>[2x]MSQRITIDPVTRIEGH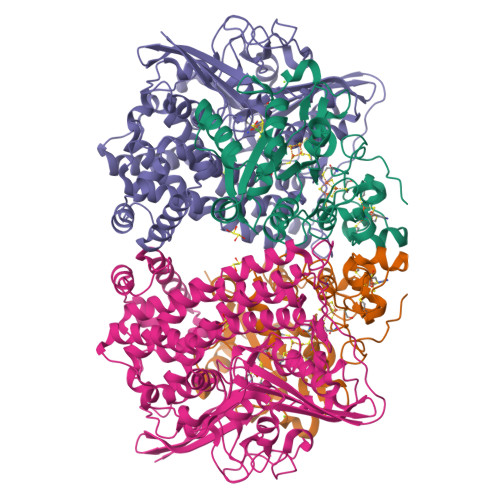LRIDCEIENGVVSKAWASGTMWRGMEEIVKNRDPRDAWMIVQRICGVCTTTHALSSVRAAESALNIDVPVNAQYIRNIILAAHTTHDHIVHFYQLSALDWVDITSALQADPTKASEMLKGVSTWHLNSPEEFTKVQNKIKDLVASGQLGIFANGYWGHPAMKLPPEVNLIAVAHYLQALECQRDANRVVALLGGKTPHIQNLAVGGVANPINLDGLGVLNLERLMYIKSFIDKLSDFVEQVYKVDTAVIAAFYPEWLTRGKGAVNYLSVPEFPTDSKNGSFLFPGGYIENADLSSYRPITSHSDEYLIKGIQESAKHSWYKDEAPQAPWEGTTIPAYDGWSDDGKYSWVKSPTFYGKTVEVGPLANMLVKLAAGRESTQNKLNEIVAIYQKLTGNTLEVAQLHSTLGRIIGRTVHCCELQDILQNQYSALITNIGKGDHTTFVKPNIPATGEFKGVGFLEAPRGMLSHWMVIKDGIISNYQAVVPSTWNSGPRNFNDDVGPYEQSLVGTPVADPNKPLEVVRTIHSFDPCMACAVH;>MEMAESVTNPQRPPVIWIGAQECTGCTESLLRATHPTVENLVLETISLEYHEVLSAAFGHQVEENKHNALEKYKGQYVLVVDGSIPLKDNGIYCMVAGEPIVDHIRKAAEGAAAIIAIGSCSAWGGVAAAGVNPTGAVSLQEVLPGKTVINIPGCPPNPHNFLATVAHIITYGKPPKLDDKNRPTFAYGRLIHEHCERRPHFDAGRFAKEFGDEGHREGWCLYHLGCKGPETYGNCSTLQFCDVGGVWPVAIGHPCYGCNEEGIGFHKGIHQLANVENQTPRSQKPDVNAKEGGHHHHHH[2x]>QGMQTIHIGVLSASDRASK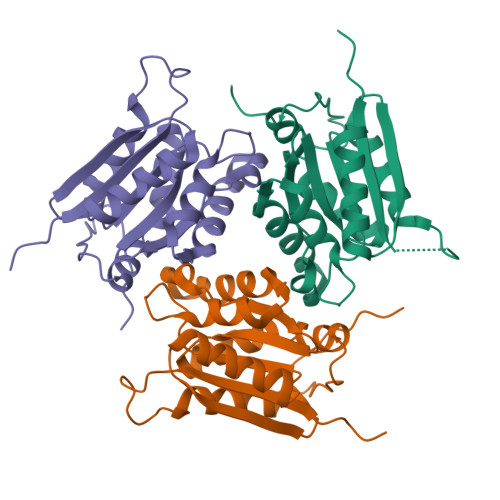GVYEDLSGKAIQEVLSEYLLNPLEFHYEIVADERDLIEKSLIKMCDEYQCDLVVTTGGTGPALRDITPEATKKVCQKMLPGFGELMRMTSLKYVPTAILSRQSAGIRNKSLIINLPGKPKSIRECLEAVFPAIPYCVDLILGNYMQVNEKNIQAFRPKQ[6x]>[2x]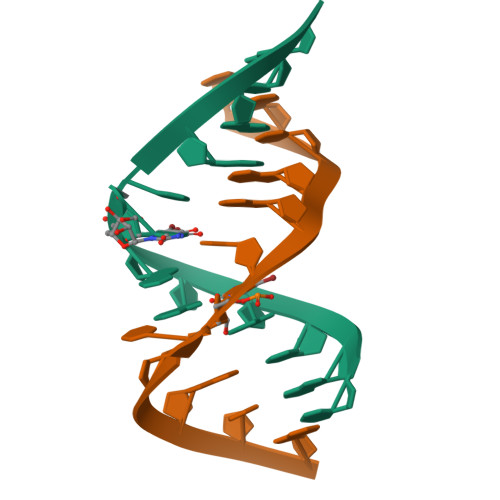CGCGAAUXAGCG1(S)-AMINOETHYL-(2-CARBOXYPROPYL)PHOSPHORYL-PHOSPHINIC ACID | C6 H15 N O7 P2 | 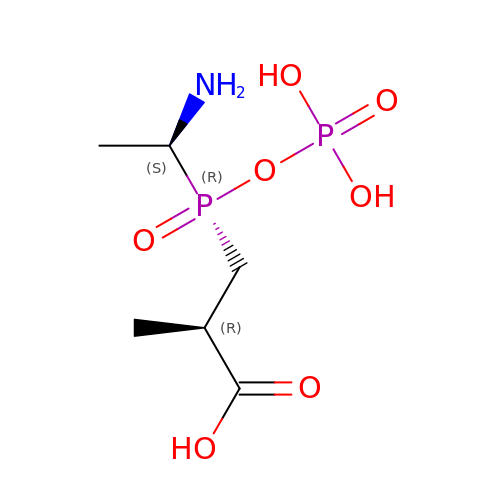BAIYWTZQRMCJBV-DKDXWZAISA-N>MEDKGKTFFGQPLGLSTLFMTEMWERFSYYGMRAILLYYMWFLISTGDLHITRATAASIMAIYASMVYLSGTIGGFVADRIIGARPAVFWGGVLIMLGHIVLALPFGASALFGSIILIIIGTGFLKPNVSTLVGTLYDEHDRRRDAGFSIFVFGINLGAFIAPLIVGAAQEAAGYHVAFSLAAIGMFIGLLVYYFGGKKTLDPHYLRPTDPLAPEEVKPLLVKVSLAVAGFIAIIVVMNLVGWNSLPAYINLLTIVAIAIPVFYFAWMISSVKVTSTEHLRVVSYIPLFIAAVLFWAIEEQGSVVLATFAAERVDSSWFPVSWFQSLNPLFIMLYTPFFAWLWTAWKKNQPSSPTKFAVGLMFAG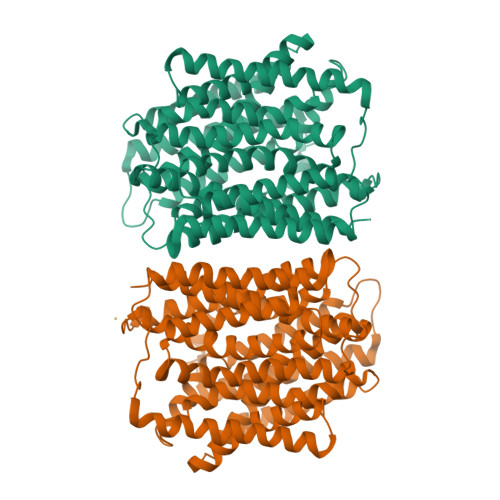LSFLLMAIPGALYGTSGKVSPLWLVGSWALVILGEMLISPVGLSVTTKLAPKAFNSQMMSMWFLSSSVGSALNAQLVTLYNAKSEVAYFSYFGLGSVVLGIVLVFLSKRIQGLMQGVEGSENLYFQ[2x]>[2x]MAHHHHHHM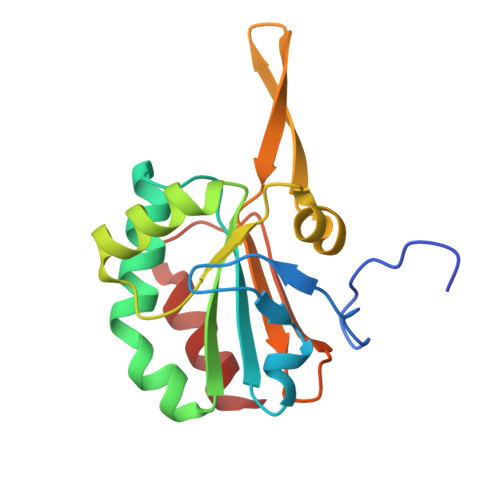SVEVDRQVPDFTAPATGGDISLSDLKGRKLVLYFYPKDNTPGCTTEGLQFRELYPKFKKAGAEIIGVSRDSLRSHDNFKAKLELPFPLISDADEALCALFDVIKMKKMYGKEVRGIERSTFLIDADGVLRQAWRGIKVPGHVDDVLSAVQAL>[6x]MLYVYMDGEFVPENEAKVSIFDHGFLYGDGVFEGIRAYNGRVFRLKEHIDRLYDSAKAIDLEIPITKEEFMEIILETLRKNNLRDAYIRPIVTRGIGDLGLDPRKCQNPSIIVITKPWGKLYGDLYEKGLTAITVAVRRNSFDALPPNIKSLNYLNNILAKIEANAKGGDEAIFLDRNGYVSEGSGDNIFVVKNGAITTPPTINNLRGITREAVIEIINRLGIPFKETNIGLYDLYTADEVFVTGTAAEIAPIVVIDGRKIGDGKPGEITRKLMEEFSKLTESEGVPIYE

Branched chain TAms (BCATs) catalyse reversible transamination of branched chain amino acids. The subunit of the archaeal BCATs has a PLP type IV fold typical of other BCATs, D-amino acid TAms and (R)-selective ωTAms and consists of two α/β domains, a small domain and a large domain connected by two inter-domain loops. A dimer formation is required for the BCAT catalytic activity, since residues from both subunits in the dimer contribute to the active site.

The AF0933 structure has been determined in the holoform (AF0933_holo) and in complex with the inhibitor gabaculine (GABC) (AF0933_GABC) to 2.1 and 2.0 Å resolution, respectively, in the orthorhombic P212121 space group. The asymmetric unit contains a hexameric AF0933 molecule which is very similar to GEO1900 hexamer observed in the crystal. The interdomain loop could only be fully built in one subunit (D) out of the six subunits in both the AF0933_holo and AF0933_GABC structures. The crystal contacts in AF0933 appear to be contributing to the lower disorder of the loop in the D subunit. The residues Gln107 and Asn108 were modeled with alternative conformations of the main chain in most subunits of the AF0933_holo structure and in the subunits E and F of the AF0933_GABC structure. Residue Glu249 is a Ramachandran plot outlier in all subunits of both AF0933 structures. In the AF0933 BCAT enzyme this loop is poorly ordered and moves away from the active site. However, the AF0933 enzyme had a native molecular mass of approximately 220 kDa as determined by size exclusion chromatography, indicating that it forms a homo-hexamer with only small amounts of a homo-dimeric enzyme observed. The AF0933 is predominantly hexameric in solution which may account for its increased thermal optimum over that of GEO1900. The AF0933 TAm subunit forms up to 27 ion pairs, with five 3-amino acid salt bridge clusters formed.> VIVTRSGAILPKPVKMSFGLLRV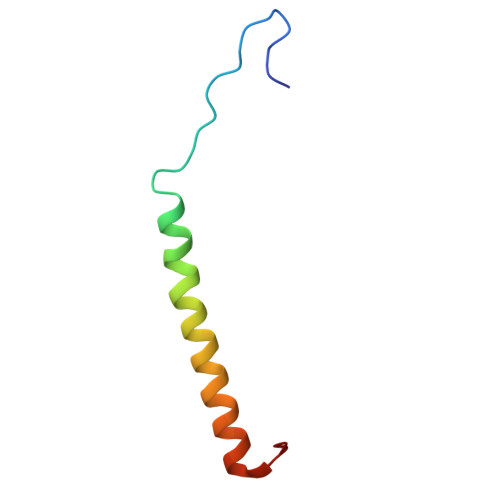FSIVIPFLYVGTLISKNFAALLEEHDIFVPE>[2x]MQVETWNAAELVAKDIAHHLHPLTNLYQLRREGPLVLVRGEGVWVWDAEGKRYLDGFAGLWNVNIGHGRRELAEAAREQMERVAFVPTFFGLASPPTIELAARLAELFPGPLDHFQFTSGGAESNETAIKIARYYWWLKGQPERVKILSRRMAYHGIAMGALSATGVPAYWEGFGPRPPGFIHLTAPYKYRFGEGLTDEEFVARLVQELEETIEREGSETIAAFIGEPVQGAGGVVVPPDGYWPAIAAVLRKYGILLILDEVITGFGRTGTLFGMQQYGVQPDIVTFAKGITSGYVPLGGVGVSDEIAETLASADRVFMHGFTYSGHPVACAVALRNLDILLAERLWENAAASGAYLLQELKRLEERPYVGEVRGKGLMLLVEVVRDKASKEKFPPEFKLGPKLEAATRRRGIIVRCTPDGIVMAPPLTISRAECDVLIEGVAAALSDVLD

Transaminases reversibly catalyze the transfer reaction of an amino group from an amine donor to a carbonyl acceptor, mediated by pyridoxal 5′-phosphate (PLP) as a cofactor. Based on the sequence information of Vf-ωTA, a novel thermostable (S)-specific transaminase from Thermomicrobium roseum (Tr-ωTA) was also identified that exhibits diverse substrate specificity and thermostability. Herein, we report the crystal structure of Tr-ωTA at 1.8 Å resolution to clarify the substrate recognition mechanism of (S)-enantioselective Tr-ωTA. The overall structure constitutes a homodimer, with each subunit comprising a large and a small domain.

The structure of Tr-ωTA was determined in the PMP-bound form at 1.8 Å resolution. In the crystal structure of Tr-ωTA, the cofactor molecule did not link to either the Lys289 residue or a possible substrate, suggesting that the cofactor was PMP. In our structure, PMP was observed only in subunit B. This finding raised the possibility that conformational differences might exist between the two subunits of Tr-ωTA. As a result, although the PMP molecules were discriminatorily distributed between the subunits in the crystal, this did not cause any structural differences in the dimer form. As PMP is present only in subunit B in the crystal structure, our crystal therefore likely constituted a mixture of the apo and holo forms of Tr-ωTA. Specifically, the oxygen atoms in the phosphate group of PMP are coordinated to adjacent water molecules and residues such as Gly121, Ala122, and Thr323. The nitrogen atom on the PMP ring forms a hydrogen bond with Asp260. Notably, Thr323 and Tyr324 from the other subunit contribute to the stabilization of the PMP position. For Tr-ωTA, Y154 along with L23 and F89 from the other subunit constitute the P-pocket components, whereas W61 and I263 are involved in the formation of the O-pocket. In contrast, the loop covering the active site of Tr-ωTA exhibited high B-factor values, suggesting that this loop likely manifests intrinsic flexibility.>[6x]HMTTADVSYLTDQGPGSGRRVPARSWLHSDAPALSLNGDWRFRLLPAAPGTAGAGSVLPSGETVEGVAAESYDDAAWDTLPVPSHWVMGQDGKYGRPIYTNVQYPFPIDPPHVPDANPTGDFRRRFDVPAQWFESTTAALTLRFDGVESRYKVWVNGQEIGVGSGSRLAQEFDVSDALRAGSNLLVVRVHQWSAASYLEDQDQWWLPGIFRDVTLQARPAGGITDAWLRTGWSARSGAGTGTIDPEITADATAFPVTLSVPELGVNVTWKSAEEVAPLALENVEPWSAEVPRLYEASVSSAAESISVRLGFRTVRIVGDQFLVNGRRVVFHGVNRHETHPDRGRVFDEAGAREDLALMKRFNVNAIRTSHYPPHPRLLDLADEMGFWVILECDLETHGFEAGGWVENPSDVPAWRDALVDRMERTVERDKNHPSIVMWSLGNESGTGSNLAAMAAWAHARDSSRPVHYEGDYTGAYTDVYSRMYSSIPETDSIGRNDSHALLLGCDSAESARQRTKPFILCEYVHAMGNGPGAMDQYEALVDKYPRLHGGFVWEWRDHGIRTRTAEGMEFFAYGGDFGEVVHDSNFVMDGMVLSDSTPTPGLYEFKQIVSPIRLGLSLPAGGKPTLAVANLRHTADASDVVLRWRVEHDGAVAASGEVAAEGSDGPLRAGESATIALPAMPAAPLGETWLTVEAVLRDATGWAPAGHPLGAVQLDLSAPAVPTRSPRPATPLDGALPVSLGPATFDAGTLVSLAGQPVSGPRLELWRAPTDNDRGAGFGAYGPGDPWLNSGRGVPAPSSE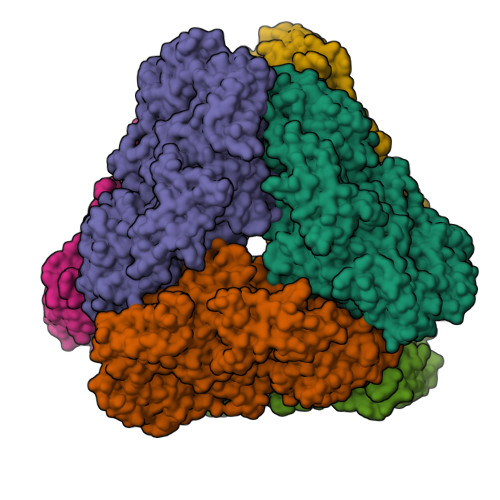AVWKQAGLDRLTRRVEDVAALPDGIRVRTRYAAADSTHSVAVEENWQLDGGELCLRIDITPSAGWNLVWPRIGVRWDLPTDVDGAAWFGAGPRESYPDSMHATMVARHAASLEELNVPYARPQETGHRSDVRWLELDRAGAPWLRIDAEPDAAGRRPGFSLARHTAQEIAAAGHPHELPTPSHSYLYVDAAQHGLGSRACGPDVWPDFALRPEARTLKLRISPA> DNPPWAKPFELLVSFLNTPKYGTFDPTPVVPVFFPFWFGMIVGDIGYALLFYLVGRWLSGYVKRNEPLVIDLFALKLKPQVIG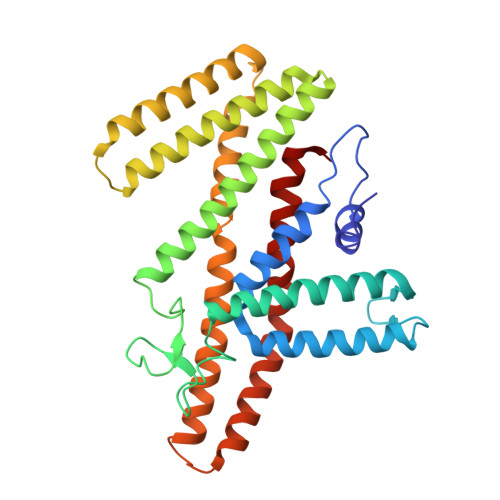KLVHILNWMVFWTVVWGVIYGEFFGTFLEHLGVFGTPEHPGLIPILIHRIDTAKTANLLILLSVAFGVVLVFFGLALRAYLGLKHRHMAHFWEGVGYLGGLVGVLALAASYLGNLQAGWLQGLMYLGFGVFLLAVLMSRIWLMIPEIFTQAGHILSHIRIYAVGAAGGILAGLLTDVGFALAERLGLLGVLLGLLVAGVLHLLILLLTTLGHMLQPIRLLWVEFFTKFGF>MLAILYDRIRPDERMLFERAEALGLPYKKVYVPALPMVLGERPKELEGVTVALERCVSQSRGLAAARYLTALGIPVVNRPEVIEACGDKWATSVALAKAGLPQPKTALATDREEALRLMEAFGYPVVLKPVIGSWGRLXXXXXXXXXXXXXXXXKEVLGGFQHQLFYIQEYVEKPGR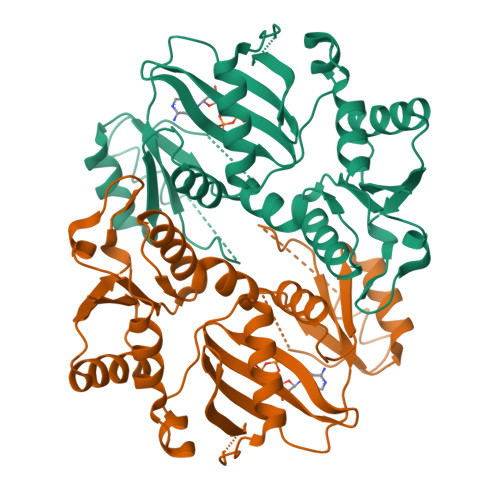DIRVFVVGERAIAAIYRRSAHWITNTARGGQAENCPLTEEVARLSVKAAEAVGGGVVAVDLFESERGLLVNEVNHTMEFKNSVHTTGVDIPGEILKYAWSLAS[2x]> MSLIHPDTAKYPFKFEPFLRQEYSFSLDPDRPICEFYNSREGPKSCPRGPLCPKKHVLPIF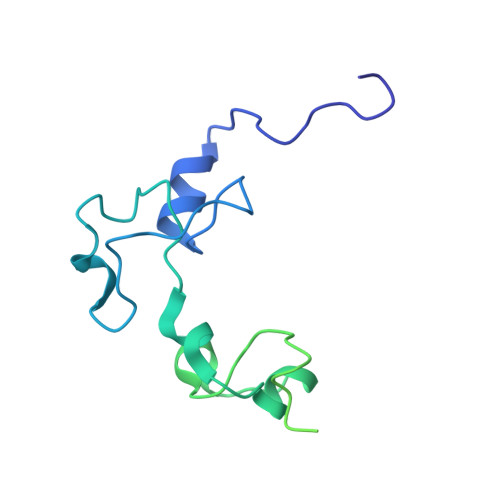QNKIVCRHWLRGLCKKNDQCEYLHEYNLRKMPECVFFSKNGYCTQSPDCQYLHIDPASKIPKCENYEMGFCPLGSSCPRRHIKKVFCQRYMTGFCPLGKDECDMEHPQFIIPDEGSKLRIKRDDEINTRKMDEEKERRLNAIINGEV>SNAMVNQLEMLYEGKAKKIYATDKEDMVIVHYKDDATAFNGEKKAQIESKGVLNNEITSLIFEMLNKEGIKTHFVEKLNDRDQLCKKVEIVPLEVIVRNVAAGSMAKRLGLEEGYELKTTVFELSYKDDSLGDPLINDYHAVGIGATTFEELNKIYEITAKVNEILKEAFKKQNINLIDFKLEFGRYNGEILLADEISPDTCRFWDATTGEKMDKDRFRRDMGNVIN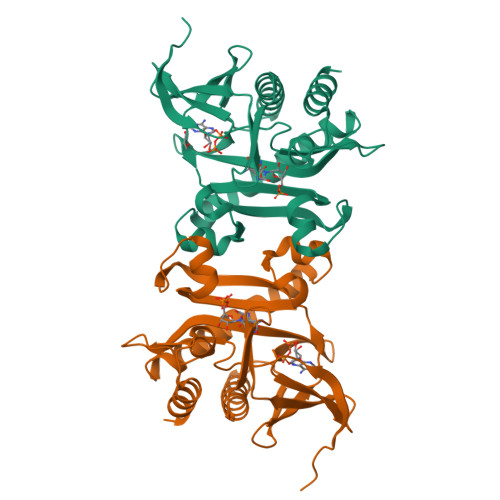GYREVLNRLRN[2x]>[2x]SNAMSKMIAVTMGDPAGIGPEIIIKSLAEGALSGAPVVVVGCAQTLRRILALNITPRAELRIIDHPAEASFSPATINVIDEPLSDPQGLRPGEVQAQAGDLAFRCI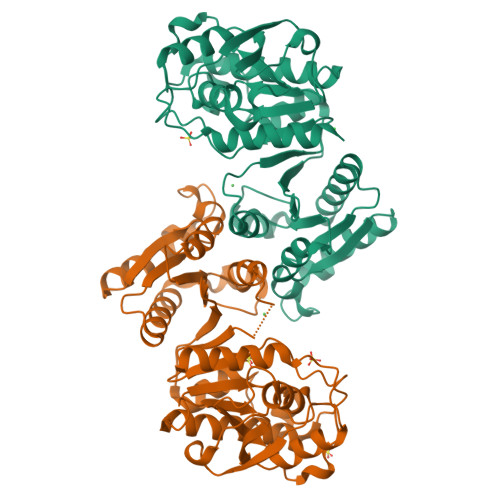RRATALALEGAVAAIATAPLNKEALHLAGHAYPGHTELLAHLTQTTDYAMVLYTEKLKVIHITTHISLRQFLDTLNQPRIETVIGVADRFLRRVGYPRPRIAVAGVNPHAGENGLFGDEEIRIVAPAVAAMRAKGVEVTGPCPPDTVFMQCHEGMYDMVVAMYHDQGHIPLKLLGFYDGVNITAGLPFIRTSADHGTAFDIAWTGKAKSESMATSIELAMHIAQE>MDHLPIFCQLRDRDCLIVGGGDVAERKARLLLEAGARLTVNALTFIPQFTVWANEGMLTLVEGPFDETLLDSCWLAIAATDDDTVNQRVSDAAESRRIFCNVVNAPKAASFIMPSIIDRSPLMVAVSAGGTSPVLARLLREKLESLLPQHLGQVARYAGQLRARVKKQFATMGERRRFWEKFFVNDRLAQSLANADEKAVNATTERLFSEPLDHRGEVVLVGAGPGDAGLLTLKGLQQIQQADIVVYDRLVSDDIMNLVRRDADRVFVGKRAGYHCVPQEEINQILLREAQKGKRVVRLKGGDPFIFGRGGEELETLCHAGIPFSVVPGITAASGCSAYSGIPLTHRDYAQSVRLVTGHLKTGGELDWENLAAEKQTLVFYMGLNQAATIQEKLIAFGMQADMPVALVENGTSVKQRVVHGVLTQLGELAQQVESPALIIVGRVVALRDKLNWFSNH[2x]

Siroheme is the modified isobacteriochlorin tetrapyrrole used by siroheme-dependent sulfite and nitrite reductases (SiR/NiRs) in catalyzing the six-electron reduction of sulfite to sulfide or nitrite to ammonia. CysG is encoded by a gene fusion between a C-terminal SUMT (CysGA) and an N-terminal bifunctional dehydrogenase/ferrochelatase (CysGB). The N-terminal enzyme module, CysGB, is a three-domain bifunctional dehydrogenase/ATP-independent class III ferrochelatase12 that performs the final two steps of siroheme biosynthesis. The C-terminal enzyme module, CysGA, is homologous to a well-studied class of SAM-dependent uro’gen III methyltransferases (SUMTs) that catalyzes the methylations to generate precorrin-210,13.

D104 has been implicated in its chelatase activity but its exact role is unknown. Alteration to asparagine results in an enzyme with a severe growth defect, 10-fold lower dehydrogenase activity, and 200-fold lower chelatase activity. The D104N variant is also sensitive to addition of Co2+, but with the same dose–response as CysG. The D104A and D104N structures were determined to ensure that there were no gross structural defects that arose from the alterations that might impact their function. Indeed, both altered enzymes were crystallized and the structures are largely similar to Met8p. The asparagine side chain is pointed away from the tetrapyrrole binding pocket, toward the Rossmann fold, as D104 does in the apo structure. Presumably, in the D104N altered CysG, the asparagine can reorient and partially act in the same capacity as the aspartic acid in catalyzing dehydrogenation and chelation. Asparagine rarely serves as a nucleophile, but there are some examples of proteases that use an asparagine in this capacity, so it may be sufficient to allow basal catalysis. It may also be sufficient to coordinate the water molecule that is poised over the tetrapyrrole nitrogens to prepare the tetrapyrrole for metal insertion, albeit less efficiently than the aspartate. As regards metal ion specificity, however, D104N is no more sensitive to increasing cobalt dose than CysG, suggesting that metal ion specificity does not depend entirely on the nature of the ligand that recruits the metal to the tetrapyrrole.>MHHHHHHHGMHHHHHHHGSPKDLTIPTGADGEGSVQVHLDEADKITGAKVFAVYGKGGIGKSTTSSNLSAAF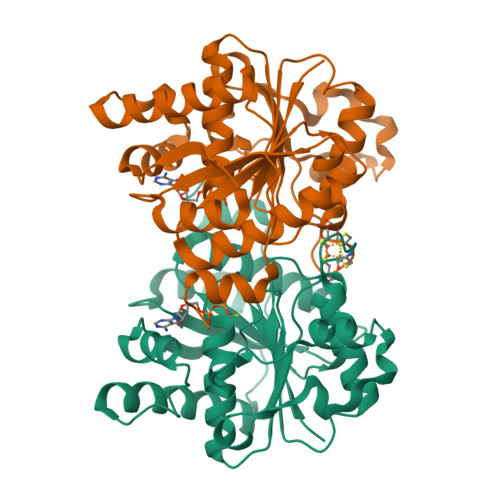SILGKRVLQIGCDPKHDSTFTLTGSLVPTVIDVLKDVDFHPEELRPEDFVFEGFNGVMCVEAGGPPAGTGCGGYVVGQTVKLLKQHHLLDDTDVVIFDVLGDVVCGGFAAPLQHADQAVVVTANDFDSIYAMNRIIAAVQAKSKNYKVRLAGCVANRSRATDEVDRFCKETNFRRLAHMPDLDAIRRSRLKKKTLFEMDEDQDVLAARAEYIRLAESLWRGLDPIDPHSLPDRDIFELLGFD[2x]> SMQASRARLFKEYKEVQREKVADPDIQLICDDTNIFKWTALIKGPSETPYEGGVFQLAFSVPEPYPLQPPQVRFLTKIFHPNVHFKTGEICLDILKNAWSPAWTLQSVCRAIIALMAHPEPDSPLNCDSGNLLRSGDVRGFNSMAQMYTRLAAMPKKGLEVLFQ;> GPAVQDVVDQFFQPVKPTLGQIVRQKLSEGRKVTCRLLGVILEETSPEELQKQATVRSSVLEVLLEITKYSDLYLMERVLDDESEAKVLQAL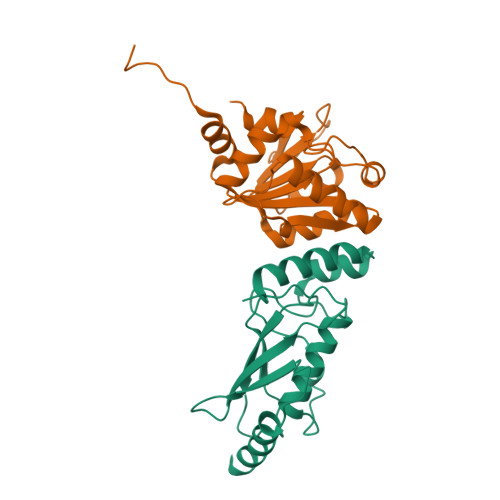ENAGVFTSGGLVKDKVLFCSTEIGRTSFVRQLEPDWHIDTNPEISTQLARFIKYQLHVATVKPERTAPNVFTSQSIEQFFGSV2-{(S)-(2-chlorophenyl)[2-(4,4-difluoropiperidin-1-yl)ethoxy]methyl}-1H-pyrrolo[3,2-b]pyridine-7-carboxylic acid | C22 H22 Cl F2 N3 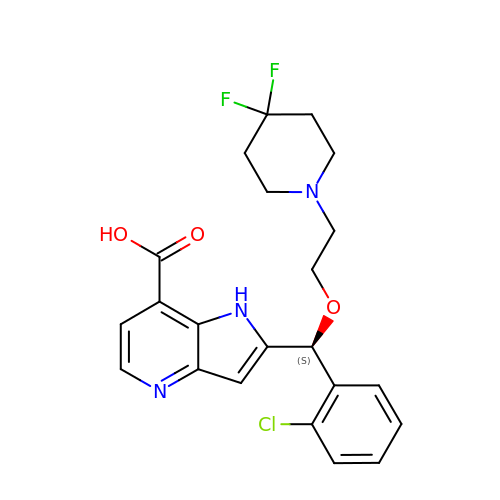O3 | QCUMGQXPGZQHID-FQEVSTJZSA-N>[2x]GSHMEEKY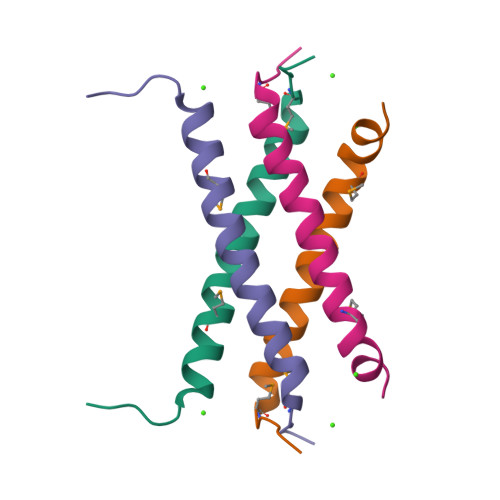YMDADLLREIKQHLKQQQEGLSHLMSIIKDDLEDIKLV> SMDL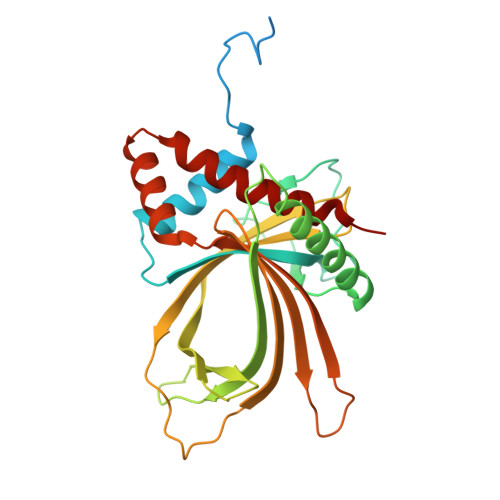KGLLHEENELPSIEKRKIDENAVEHDKVERKRTKSVAVPKIEMNFLNKPIVPDTTKVISNFLTHYLITEPVEHVEIEAKLGTLIDLETQNRFEFPVMNETILNPEFNLRTRFESDMTASEHKYLNEFLNQAFRDSQKPGRLPFAYKHTKQVDLFYETEDNSRDKIRVSKNQSDNQVLACVKKRRVADLFLYCPNDAFDIRISISDELPVSMPSGNQQPSLTRLKDRVGYVHQEIKIDLTKTTQNDPVYDTTERHELEVEFGNIADLRDRAQKAKDGMEAPLFRRVQLFMDNVRILRREHS> GPGSMEASCLELALEGERLCKSGDCRAGVSFFEAAVQVGTE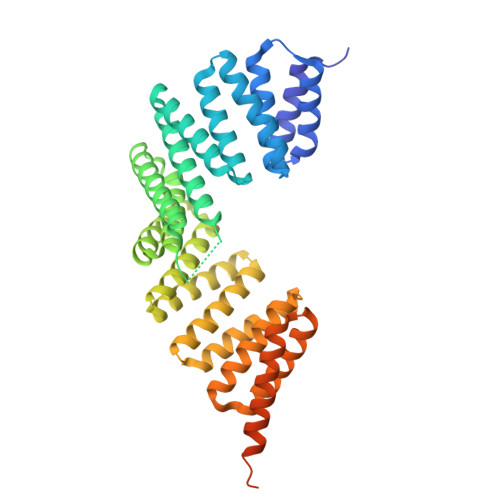DLKTLSAIYSQLGNAYFYLHDYAKALEYHHHDLTLARTIGDQLGEAKASGNLGNTLKVLGNFDEAIVCCQRHLDISRELNDKVGEARALYNLGNVYHAKGKSFGCPGPQDVGEFPEEVRDALQAAVDFYEENLSLVTALGDRAAQGRAFGNLGNTHYLLGNFRDAVIAHEQRLLIAKEFGDKAAERRAYSNLGNAYIFLGEFETASEYYKKTLLLARQLKDRAVEAQSCYSLGNTYTLLQDYEKAIDYHLKHLAIAQELNDRIGEGRACWSLGNAYTALGNHDQAMHFAEKHLEISREVGDKSGELTARLNLSDLQMVLGLSYSTNNSIMSENTEIDSSLNGVRPKLGRRHSMENMELMKLTPEK> MGSDSIDTPNYDVQKHINKLCGMLLITEDANHKFTGLIGMLYAMSRLGREDTIKILRDAGYHVKANGVDVTTHRQDINGKEMKFEVLTLASLTTEIQINIEIESRKSYKKMLKEMGEVAPEYRHDSPDCGMIILCIAALVITKLAAGDRSGLTAVIRRANNVLKNEMKRYKGLLPKDIANSFYEVFEKHPHFIDVFVHFGIAQSSTRGGSRVEGIFAGLFMNAYGLEHHHHHH;> MGSDSIDTPNYDVQK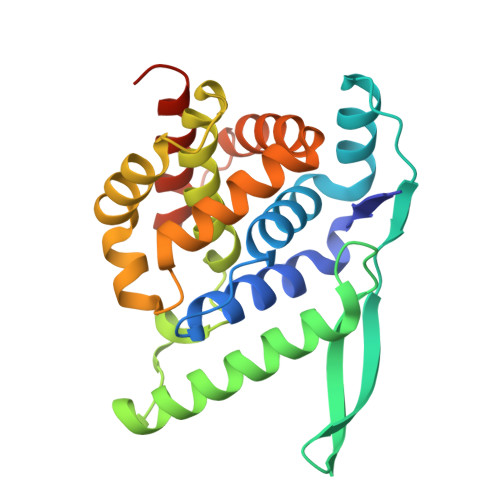HINKLCGMLLITEDANHKFTGLIGMLYAMSRLGREDTIKILRDAGYHVKANGVDVTTHRQDINGKEMKFEVLTLASLTTEIQINIEIESRKSYKKMLKEMGEVAPEYRHDSPDCGMIILCIAALVITKLAAGDRSGLTAVIRRANNVLKNEMKRYKGLLPKDIANSFYEVFEKHPHFIDVFVHFGIAQSSTDGGSRVEGIFAGLFMNAYGLEHHHHHH> XMEQLSTANTHFAVDLFRALNESDPTGNIFISPLSISSALAMIFLGTRGNTAAQVSKALYFDTVEDIHSRFQSLNADINKPGAPYILKLANRLYGEKTYNFLADFLASTQKMYGAELASVDFQQAPEDARKEINEWVKGQTEGKIPELLVKGMVDNMTKLVLVNAIYFKGNWQQKFMKEATRDAPFRLNKKDTKTVKMMYQKKKFPYNYIEDLKCRVLELPYQGKELSMIILLPDDIEDESTGLEKIEKQL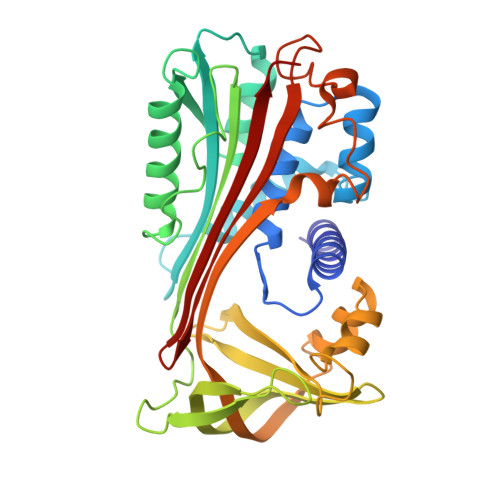TLDKLREWTKPENLYLAEVNVHLPRFKLEESYDLTSHLARLGVQDLFNRGKADLSGMSGARDLFVSKIIHKSFVDLNEEGTEAAAATAGTILLA V. vulnificus secretes a large multifunctional-autoprocessing repeats-in-toxin (MARTX) as a main virulence factor via an atypical type I secretion system. The central region of the MARTX toxin of V. vulnificus MO6-24/O contains an autoprocessing cysteine protease domain (CPD) and four effector domains including the domain of unknown function (DUF1), the Rho-inactivating domain (RID), an αβ hydrolase (ABH), and makes caterpillars floppy-like domain (MCF). The CPD directs the proteolytic processing of effector modules after activation by binding to the eukaryotic cell-specific inositol hexakisphosphate (InsP6). The V. vulnificus MARTX CPD displays a canonical CPD structure with the central seven-stranded β-sheet flanked by three α helices.

To examine the structure of the processed CPD, we purified the wild-type CPD lacking the N-terminal autocleavage sequence (post-CPD, residue 3592–3796). The post-CPD construct in the absence of InsP6 was susceptible to proteolytic degradation of the C-terminal β-flap during protein expression and purification. We obtained the crystals in a week at room temperature and determined the structure of the post-CPD at 2.2 Å resolution. However, the C-terminal β-flaps (residues 3762–2796) were not visible. In the asymmetric unit of crystals, there were two CPD molecules coordinating a single molecule of InsP6 in the center of the non-crystallographic two-fold axis. Considering the proteolytic susceptibility of the β-flap, it seems that the crystals were formed by proteolyzed fragments lacking the β-flap (post-CPD Δβ-flap) or that the β-flaps were completely disordered. A single molecule of InsP6 in the crevice of the dimer interface interacts with the four basic residues of the InsP6-binding pockets from each protomer. Compared to the structure of the pre-CPD-InsP6 complex, the position of InsP6 in the post-CPD Δβ-flap was shifted 3 Å away from the binding pocket to share the coordination of a single InsP6 molecule by two protomers. Due to the lack of interaction between the β-flap and the β7-α3 loop, the catalytic residue Cys3727 is displaced 5.4 Å toward the helix α1, occluding the substrate binding pocket. Though the dimeric structure of the post-CPD Δβ-flap is physiologically not relevant, the monomeric structure seems to represent the inactive conformation of the core CPD when InsP6 is not loaded to the post-CPD.

>[2x]GSAMGSILHNQNVNDWERVVVTPTADGGESRFDGQIIVQMENDDVVAKAAANLAGKHPESSVVVQIDSDGNYRVVYGDPSKLDGKLRWQLVGHGRDDSESNNTRLSGYSADELAVKLAKFQQSFNQAENINNKPDHISIVGCSLVSDDKQKGFGHQFINAMDANGLRVDVSVRSSELAVDEAGRKHTKDANGDWVQKAENNKVSLSWD> MNLRIPWKEVYYLGYNMGNYIKISEPELLFVLRNKPQIKDRLKLDEKTIIKEGVKKYKNFWEIYYTVKDLILRGYRVRFDGFFIELYEKGIIPGTIEQDYLVYPVSGEIRMTWGELLDIY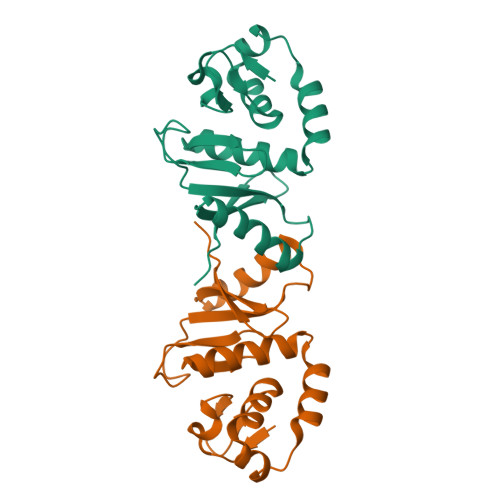NKAIARKSKFMLAIVDSEGDVTYYEFRKLRSNK> MLVDSMGDIVITNDGATILKEMDIQHPAAKMIVEVSKTQDAEVGDGTTTAA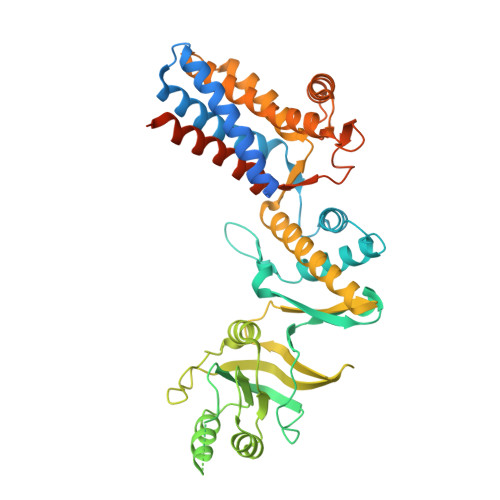VLSGELLSKAEELIMKGVHSTIISEGYRHAAEKCREILETITIAISPDDEAALIKIAGTAITGKGAEAYKEKLSALTVKAVRSIVEEEEDGLKVNVLENIKIEKRAGGSIDDSELIDGLVIDKERSHPNMPEKVENAKILLLSCPVEFRKTEVDSEIKITSPGQMQLFLDQEEKMMREMAEKVIASGANVVFCQKGIDDMAQYYIEKAGIYAVRRVKKSDLKRLSKVTGATIIQDLDQITTEDVGTAGLVEEKEVRGGKMTYVTGCQNSKAVTVLLHGGTEHVVDSLDHALNDALHVVGVVIEDGKVVVGGGSSEVELSLRLSEYASTLKGREQLAVSKFAEALEVIPVALAENAGLDPIDIMVELRSQHEKGNKNAGLNVYTGEVVDMWENDVIEPLRIKTQAINAAMEATVMILRIDDVVASKGSANQGMGPGGLPDMPDLDMDAAY>YQQRQQKVKDRVDARVAQAQEERGIIIVFTGNGKGKTTAAFGTAARAVGHGKNVGVVQFIKGTWPNGERNLLEPHGVEFQVMATGFTWETQNREADTAACMAVWQHGKRMLADPLLDMVVLDELTYMVAYDYLPLEEVISALNARPGHQTVIITGRGCHRDILDLADTVSELRPVKHA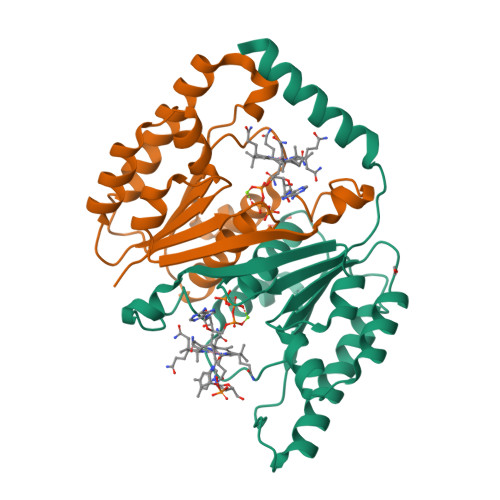FDAGVKAQMGIDY[2x]> KQTNNAPKPKFQKF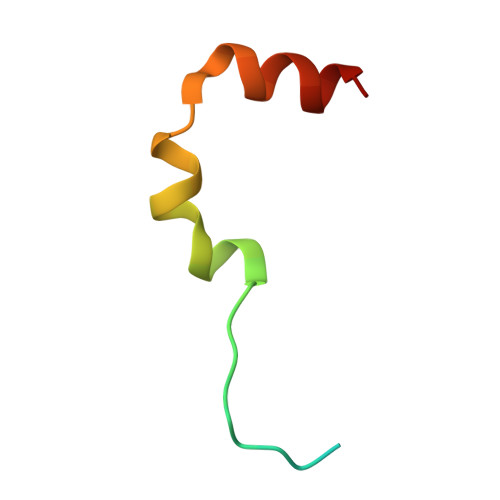LDRRRSFRDIQGAISKIDPEIIKSLLAST> GEIKGR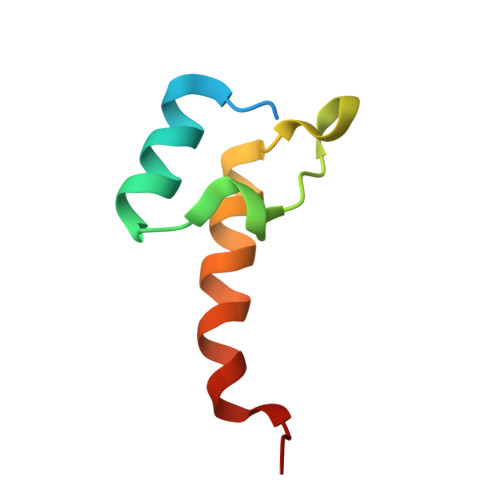KTLATPAVRNLAMENNIKLSEVVGSGKDGRILKEDILNYLEKQTLEHHHHHH>MATSPEGIWSNSGALTFEDPADDSEILFAGVRDVTITPAYEHAELYTIDSTFRDEVKRYEHNVNVEITYAKFSLEFAQEWLGGPGATATASQDDSDPMKFNLENVTPSASGGFERTTAVENVVFPELPLDSATYGEYEEYSLTGSGRSVTNLADTSGV[66x];>MVDATLSRGGTSVDIPLVEEGGEILLSSTFGKPEVNVRKSGGSLNPRVIDSWSGLQTFQLVGKLYDYSTSHQLADLVKTASTTPLELQIPQDAYPDTVTVAPAAGQASALTLEYPAGRKDLVDVSLSLTRVDPNSVRGVGDQQATTPTTTGTGPVEVTAGGTTVQLPSSGLSVERTVGRPNDAVRRVPRQADPRYEVKAKVTNDVFTFSFETLDNIPATLNALTDNVFREQLGRDGVTLDFNGLLGLGSVKAIPVGSSPFRQVHQAGRGWVTVPTLEFRRIYSNE[3x];>MPDPSIDEVSKSDWDALTTQEQDDIISQVENLSSTGWVNTSRERKAEAIRSAIAERDTLYSGNMSRLPTLDGDAEYFTLYLSAHKIQLFEGGEAQSESGEGGSVSYSTGGGGEKDLQKTRYGRMALEYVWEDNSIAALRTY[12x];>[6x]MATTSASHHVQAIIDLLEAAPDADWTPTQTPTVKRYWDDAQSERGPGADMPAILYVWSPTTSSLDRFSMDGDVFDQNDSIEVQAWSFDETEVEQLQGDIVQILSEYLDDNEVQTPYSDVAPTGTNDFREQTPARTTGHYIMSVEVETRGLSETAKNA

Here, we present the near-atomic resolution structure of Haloferax tailed virus 1 (HFTV1), an archaeal virus thriving in extreme salinity. Through single-particle analysis, we obtained near-atomic resolution maps of DNA-filled and empty virions, enabling us to assemble full atomic models of the virus pre- and post-DNA release, including all structural protein components. The full atomic structure revealed that the virus has a length of 1350 Å and an icosahedral head with a diameter of ~600 Å. The tail has a length of 560 Å and terminates into a baseplate with three radiating TFs of ~190 Å in length.

The empty structure corresponds to a postinfection state. Compared to its DNA-filled counterpart, the empty virus lacks the tape measure protein (TMP), baseplate hub (BPH), and tail fibers (TFs), indicating that these parts are jettisoned during DNA ejection. However, the length of the tail tube remains unaltered, demonstrating that it does not contract during DNA ejection, similar to siphoviruses that infect bacteria. (C) Structure of the tail of the empty virus. The dsDNA, TMP, and baseplate are missing. Instead, a density appears to plug the capsid-facing side of the portal. Otherwise, the portal and the components of the tail tube are unchanged in width, length, and conformation, indicating a rigid structure. In the empty virus, the TMP and TDS are absent, demonstrating that they are released during DNA ejection. Genome release in HFTV1 triggers structural changes in the distal tail region, including BPH detachment and TF dissociation.> MSLPAHLQQTFSPEEIQFIVENEPIKIFPRITTRQKIRGDDRGTGNHTRWQLITTDDKALNNMVAMRSTEVVLWIALLLKQQSKCSIV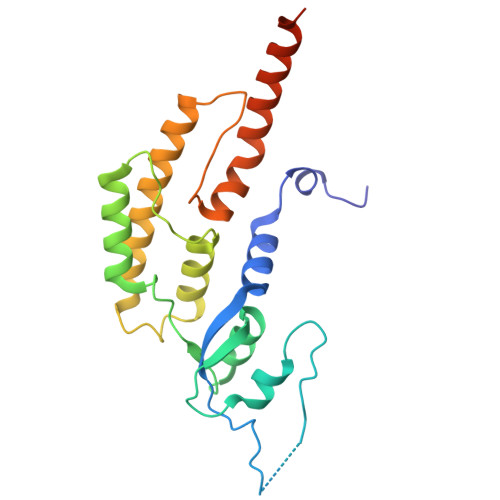APQWLTTKELDRKIQYEKTHPDRFSELPWNWLVLARILFNKAKDDFHDPIHELRGKIQDLREIRQIKVLKGLKYLNESHLQLDNLSLLEINELRPFITEIMDKLREIHTASLTAGTENDEEEFNI>MSNSKTFLSLTFFTTFLFFSFVNATYYQDISPSFLGFKQEKLTHIHFFLHDIVTGPKPTMIIASESPLNGKSESPLPFGSIVVLEDPLTVGPELNSELIGKAQGFYVTVSQAAVLELELVMGMTFVFTGGKYNGSTLSVLGRNEIISPIREMPIIGGTGEFRFARGFLQAKSHA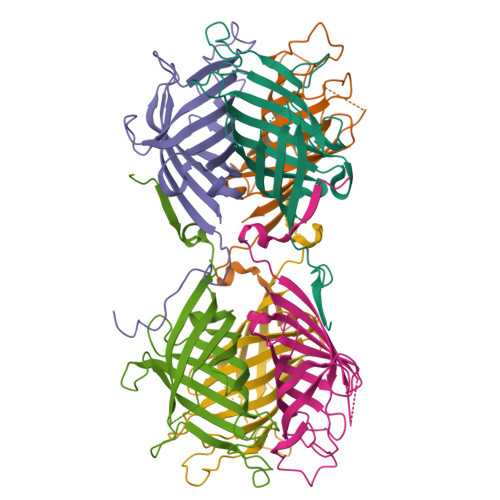VDYHEGDAHVEYNVYVFHYPSTSSSSEDFEEGSRFMKEPIFGQI[6x]> 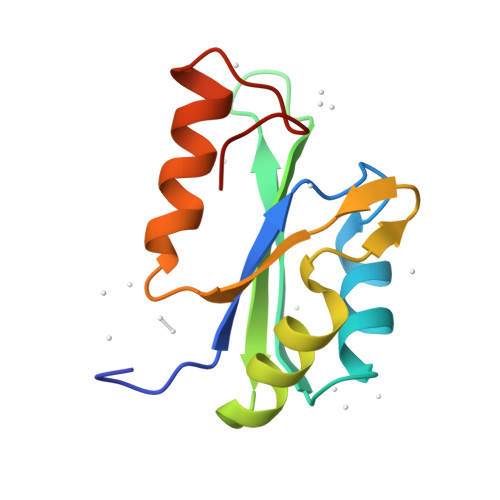GGQIPLKEVTFARLNDNVRETFLKDMCRKYGEVEEVEILLHPRTRKHLGLARVLFTSTRGAKETVKNLHLTSVMGNIIHAQLDIKGQQRMKYYELIVNGSYTPQTVPTGG>[2x]MEFYNSTNEIPEEMLKGIDLTYPQLTYLPETGILYDNTYNEKTVPIISGGGSGHEPAHVGYVGSGMLAAAVTGPLFIPPKSKNILKAIRQVNSGKGVFVIIKNFEADLKEFNE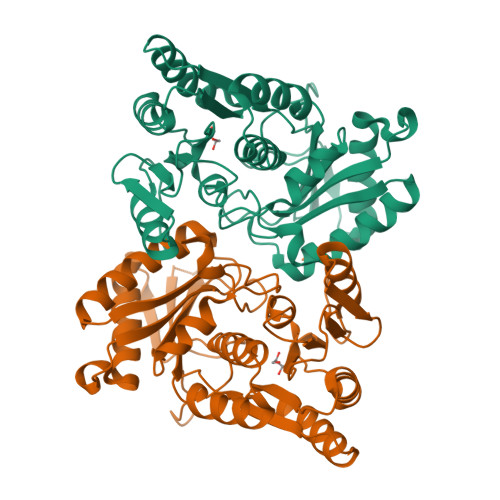AIKEARTEGIDVRYIVSHDDISVNAYNFHKRHRGVAGTILLHKILGAFAKEGGSIDEIEQLALSLSPEIYTLGVALAPVHFPHQKTSFVLAEDEVSFGIGIHGEPGYRVEKFEGSERIAIELVNKLKAEINWQKKANKNYILLVNGLGSTTLMELYSFQYDVMRLLELEGLSVKFCKVGNLMTSCDMSGISLTLCSVKDPKWLDYLNVPTGAFAWLEHHHHHH>[8x]GSHMQSDSAVLQWANQAAIAAFTYNFVNYRDELQASSGFFTAEGWDQFLGALEQSNNLDAVKAKKLVVSAVATRAPIILQKGVLNGRYSWRVQMPILVTYQSASEFTQQNNVVTMLITRVSTLNSPRGIGISQFVVGPASGGVS

DotI is a 23 kDa inner membrane protein essential for intracellular growth of L. pneumophila within mammalian and protozoan cells. DotI has one transmembrane domain in its N-terminal region, followed by a periplasmic domain13. DotI is conserved in all of the identified type IVB secretion systems, including the conjugation systems of R64 and related plasmids. Structural analysis of the periplasmic domains of DotI and its R64 ortholog TraM demonstrated that DotI and TraM are structural homologs of the T4ASS protein VirB8.

DotIC crystallized in two distinct forms (Form I and Form II) under different conditions. The structure model of Form I (space group: P21212) was refined to a resolution of 2.2 Å with the working R and the free R factor of 19.1% and 23.5%, respectively, and Form II (space group: I432) to a resolution of 3.5 Å with the working R and the free R factor of 17.9% and 21.6%, respectively. Form I and Form II contain eight and four molecules in its asymmetric unit, respectively, and the structures of these molecules are almost identical. DotIC is a single domain protein composed of four helices (α1 - α4) in one half and one β-sheet in the other half. The sheet is highly twisted at its center with an interruption in β1, therefore can be divided into two parts, Sh1 and Sh2. Sh2 comprises βs, β1a, the C-terminal half of β2 and the N-terminal half of β3, and forms a large cleft with α3 and α4. The cleft of the molecule in the Form I crystal is filled by 2-methyl-2,4-pentanediol (MPD) molecules, which is included in the mother solution for the Form I crystal. DotIC forms a stack of two octameric rings in the Form I crystal. This asymmetric unit contains eight DotIC molecules that form a head-to-head stack of two half rings composed of four monomers each. The crystallographic two-fold axis at the center of the half rings produces the two octameric rings.Rab proteins, the biggest subfamily within the superfamily of small GTPases, are major regulators of vesicular trafficking in eukaryotic cells. One such family of effector proteins that was reported to link Rab proteins and the cytoskeleton is the Mical (molecules interacting with CasL) family. In this publication, we present a thorough biochemical and structural analysis of a Rab effector domain termed bivalent Mical/EHBP Rab binding (bMERB) domain. The results show that the domains probably constitute a Rab8-effector family involved in endosomal trafficking, and the Rab-binding specificity can be well explained from the 3-dimensional structures of complexes determined in this work.

In order to understand the mode of interaction of Rab proteins and the C-terminal Rab-binding domain of Micals/EHBPs, we first aimed at determining the structure of the RBD of one member of these families. Mical-3 folds into three α-helices, the central α-helix 2 and α-helices 1 and 3 folding back on the central helix. The asymmetric unit contains two copies of Mical-3 that form a central 4-stranded coiled-coil composed of α-helices 2 and 3 of each monomer flanked by α-helices 1 on both sides. Interactions between the monomers mainly occur via two hydrophobic patches and some additional charged interactions. The dimer observed in the asymmetric unit is formed mostly by hydrophobic interactions involving the same hydrophobic patches in both monomers, and α-helices 2 and 3 from each monomer form a central 4-stranded coiled-coil. Interestingly, the Rab-binding interface in Mical-cL has a substantial overlap with the dimer interface observed in the structure of Mical-3 above. Additionally, even though all Mical constructs used have a similar molecular weight of ~18 kDa, whereas Mical-1 runs as an apparent monomer in aSEC and binding of a Rab protein induces a clear shift to higher molecular weight, both Mical-3 and Mical-cL run as apparent dimers in aSEC and binding of a Rab protein disrupts the dimer, thus not leading to a shift in retention time upon complex formation. It is however not clear at this point whether the dimer formation of Mical-3 and Mical-cL and the disruption of the dimer upon Rab-binding is of functional significance. The low affinity second binding site of Mical-3 (KD = 4.4 µM as determined by ITC) could also not be detected in these experiments, suggesting dynamic complex formation with a large koff.

>[2x]GKQEELKRLHRAQIIQRQLQQVEERQRRLEERGVAVEKALRGEAGMGKKDDPKLMQEWFKLVQEKNAMVRYESELMIFARELELEDRQSRLQQELRERMAVEDHLKTEEELSEEKQILNEMLEVVEQRDSLVALLEEQRLREREEDKDLEA>AAASFGQTKIPRGNGPYSVGCTDLMFDHTNKGTFLRLYYPSQDNDRLDTLWIPNKEYFWGLSKFLGTHWLMGNILRLLFGSMTTPANWNSPLRPGEKYPLVVFSHGLGAFRTLYSAIGIDLASHGFIVAAVEHRDRSASATYYFKDQSAAEIGDKSWLYLRTLKQEEETHIRNEQVRQRAKECSQALSLILDIDHGKPVKNALDLKFDMEQLKDSIDREKIAVIGHSFGGATVIQTLSEDQRFRCGIALDAWMFPLGDEVYSRIPQPLFFINSEYFQYPANIIKMKKCYSPDKERKMITIRGSVHQNFADFTFATGKIIGHMLKLKGDIDSNVAIDLSNKASLAFLQKHLG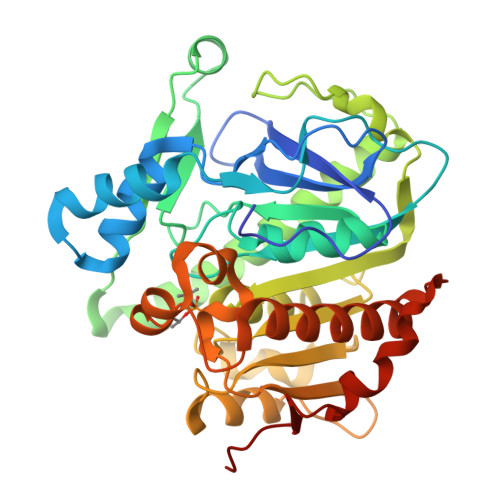LHKDFDQWDCLIEGDDENLIPGTNINTTNQHI[2x]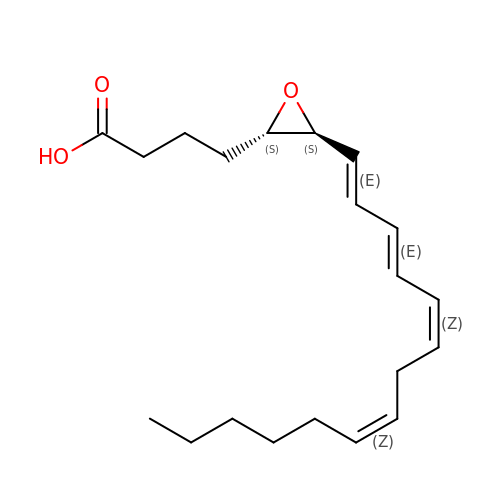5S-5,6-oxido-7,9-trans-11,14-cis-eicosatetraenoic acid | C20 H30 O3 | UFPQIRYSPUYQHK-WAQVJNLQSA-N> MDQLNALLASLEAENKQLKAKVEELLAKVG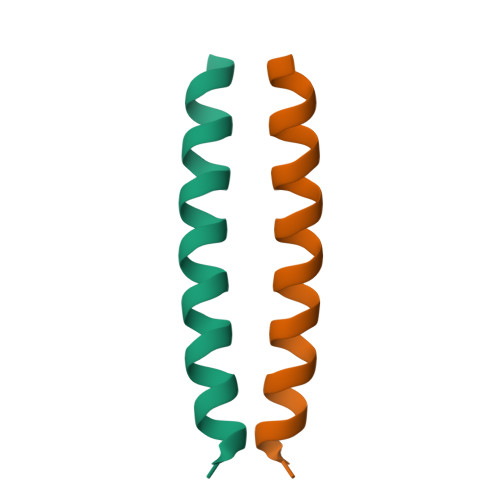E>ADNLAEFHVQNQECDSCHTPDGELSNDSLTYENTQCVSCHGTLAEVAETTKH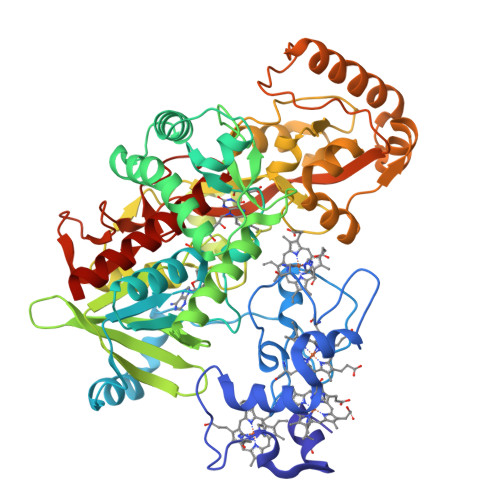EHYNAHASHFPGEVACTSCHSAHEKSMVYCDSCHSFDFNMPYAKKWLRDEPTIAELAKDKSERQAALASAPHDTVDVVVVGSGGAGFSAAISATDSGAKVILIEKEPVIGGNAKLAAGGMNAAWTDQQKAKKITDSPELMFEDTMKGGQNINDPALVKVLSSHSKDSVDWMTAMGADLTDVGMMGGASVNRAHRPTGGAGVGAHVVQVLYDNAVKRNIDLRMNTRGIEVLKDDKGTVKGILVKGMYKGYYWVKADAVILATGGFAKNNERVAKLDPSLKGFISTNQPGAVGDGLDVAENAGGALKDMQYIFAHPTLSVKGGVMVTEAVRGNGAILVNREGKRFVNEITTADKASAAILAQTGKSAYLIFDDSVRKSLSKIDKYIGLGVAPTADSLVKLGKMEGIDGKALTETVARYNSLVSSGKDTDFERPNLPRALNEGNYYAIEVTPGVHHTMGGVMIDTKAEVMNAKKQVIPGLYGAGEVTGGVHGANRLGGNAISDIITFGRLAGEEAAKYSKKN[2x]>[4x]AAGAPKPPQEPDMNNLPENPIPQHQAKFVLNTIKAVKRNREAVPFLHPVDTVKLNVPFYYNYIPRPMDLSTIERKINLKAYEDVSQVVDDFNLMVKNCKKFNGEAAGISKMATNIQAQFEKLMVKVPPKELPAGTNVA

BET proteins are chromatin-associated factors that regulate transcription and chromatin remodelling. BET proteins bind chromatin through their two BDs (BD1 and BD2), which specifically recognize histones acetylated on lysine residues. The BDs from C. albicans Bdf1 (CaBdf1) share 31–46% sequence identity with human BET BDs and 58–66% identity with those from ScBdf1 and hence are likely to bind multi-acetylated H3 and H4 tails. In conclusion, Bdf1 BDs are required for the viability and virulence of C. albicans and can be selectively targeted by small-molecule inhibitors without compromising human BET BD function.

To identify features differentiating the ligand-binding pockets of human and fungal BET BDs, we determined crystal structures for CaBdf1 BD1 and BD2. These structures exhibit the canonical BD fold (comprising helices Z,A,B and C, with the ZA and BC loops defining the ligand-binding pocket) and closely resemble those of their human BET counterparts (mean pairwise root-mean-square deviations (RMSDs) ≤1.5 Å; Supplementary Table 3). The ligand-binding loops are structurally well conserved, including nearly all water molecules implicated in ligand recognition, although the overall binding surfaces are less negatively charged in CaBdf1. Superimposing the CaBdf1 BD structures onto that of JQ1-bound Brd4 BD1 reveals no major steric clashes between JQ1 and the fungal BDs. However, whereas JQ1 fits snugly into the Brd4-binding pocket, the fit with the CaBdf1-binding pockets is poor. Replacement of Brd4 residue Leu94 by a Val or Ile residue further contributes to the poor fit. In addition, the p-chlorophenyl group of JQ1 occupies a groove in Brd4, which is absent (BD1) or shallower (BD2) in CaBdf1 (asterisks in Fig. 4c). A similar lack of complementarity between the ligand and binding pocket explains the insensitivity of CaBdf1 BDs towards PFI-1, IBET-151 and bromosporine. More generally, recognition of the four BETi compounds by human BET BDs involves 16 residues, including the eight signature residues previously used to classify human BD-binding sites. Five of these residues in BD1 and four in BD2 are invariant across human BET proteins but diverge in CaBdf1 (magenta arrows in Fig. 5), including the WPF-shelf Trp residue and the Leu residue opposite this shelf, at signature positions 1 and 3, respectively. Remarkably, nearly all of these residues have shorter side chains in CaBdf1 than in the human BET proteins, implying that selective CaBdf1 inhibition could conceivably be achieved via small molecules that clash sterically with the human, but not fungal, side chains.>[2x]MIPFKDITLADRDTITAFTMKSDRRNCDLSFSNLCSWRFLYDTQFAVIDDFLVFKFWAGEQLAYMMPVGNGDLKAVLRKLIEDADKEKHNFCMLGVCSNMRADLEAILPERFIFTEDRAYADYIYLRSDLATLKGKKFQAKRNHINRFRNTYPDYEYTPITPDRIQECLDLEAEWCKVNNCDQQEGTGNERRALIYALHNFEALGLTGGILHVNGKIVAFTFGMPINHETFG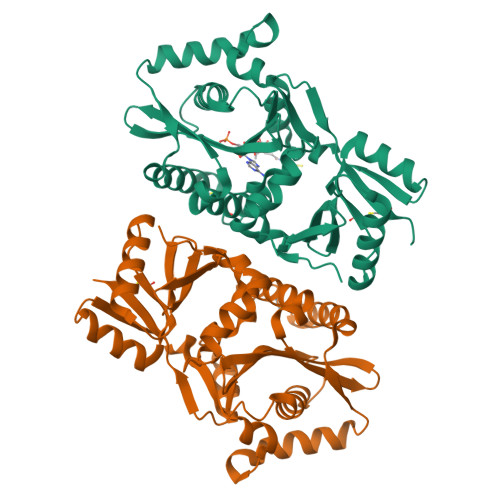VHVEKADTSIDGAYAMINYEFANRIPEQYIYINREEDLGIEGLRKAKLSYQPVTILEKYMACLKDHPMDMVRW> GHMASRAEEGLNFPTYDGKDRVVSLSEKNFKQVLKKYDLLCLYYHEPVSSDKVTQKQFQLKEIVLELVAQVLEHKAIGFVMVDAKKEAKLAKKLGFDEEGSLYILKGDRTIEFDGEFAADVLVEFLLDLIEDPVEIISSKLEVQAFERIEDYIKLIGFFKSEDSEYYKAFEEAAEHFQPYIKFFATFDKGVAKKLSLKMNEVDFYEPFMDEPIAIPNKPYTEEELVEFVKEHQRPTLRRLRPEEMFETWEDDLNGIHIVAFAEKSDPDGYEFLEILKQVARDNTDNPDLSILWIDPDDFPLLVAYW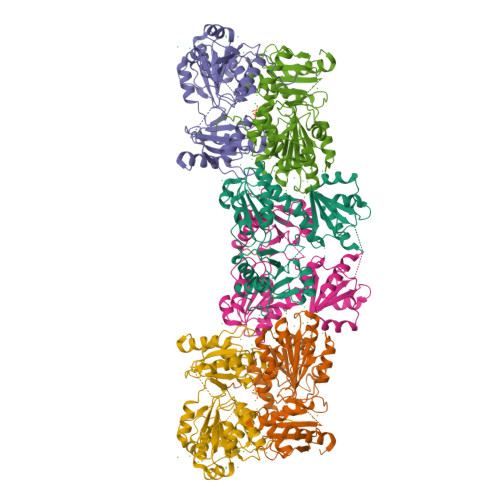EKTFKIDLFRPQIGVVNVTDADSVWMEIPDDDDLPTAEELEDWIEDVLSGKINTEDDDEDDDDDDNSDEEDNDDSDDDDDE>[2x]MSARMDNDTAALLERIRSDWARLNHGQGPDSDGLTPSAGP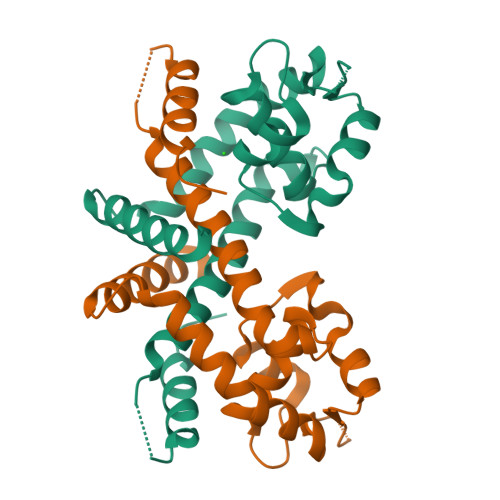MLTLLLLERLHAALGREIERTYAASGLNAAGWDLLLTLYRSAPPEGLRPTELSALAAISGPSTSNRIVRLLEKGLIERREDERDRRSASIRLTPQGRALVTHLLPAHLATTQRVLAPLSAQEQRTLEELAGRMLAGLEQGV>[2x]GAMGSMVLGKVKSLTISFDCLNDSNVPVYSSGD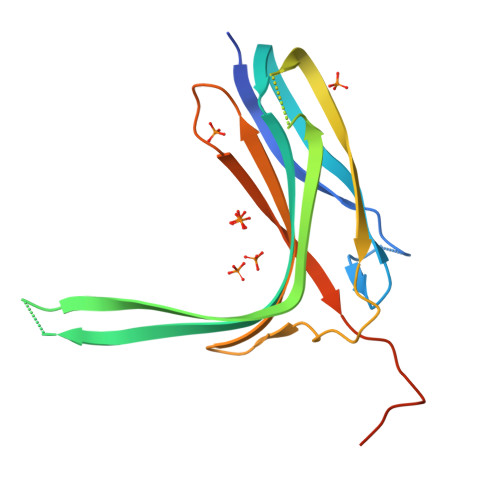TVSGRVNLEVTGEIRVKSLKIHARGHAKVRWTESRNAGSNTAYTQNYTEEVEYFNHKDILIGHERDDDNSEEGFHTIHSGRHEYAFSFELPQTPLATSFEGRHGSVRYWVKAELHRPWLLPVKLKKEFTVFEHIDINTPSLLSPQAGTKEKT N self-assembles into a helical capsid that accommodates the RNA genome to form a nucleocapsid, which protects the viral genome from host nucleases and serves as the template for viral replication. Both genome transcription and replication are carried out by the viral RNA-dependent RNA polymerase L and require the phosphoprotein P that bridges between the nucleocapsid and the polymerase. By obtaining atomic models for the authentic mumps virus nucleocapsid, we elucidate a concomitant conformational change that exposes the viral genome to its replication machinery. On the structural level, MuV nucleocapsids are templates for both viral transcription and replication.

Here, we isolated the authentic MuV nucleocapsids from stressed cells. After 1 h of 0.5 mM As(III) treatment, the isolated nucleocapsids were curved, similar to their intracellular morphology at early time points of stress but straightened on addition of the RNA-mimicking molecule heparin. We obtained two maps from subtomogram averaging on the heparin-straightened nucleocapsids isolated from cells after 1 h of 0.5 mM As(III) stress. The two maps exhibited distinctly different helical parameters: a 5.58 nm long-pitch structure constituting the majority class (77.7%) was resolved to 4.5 Å and a 4.70 nm short-pitch class (21.3%) was resolved to 6.3 Å. The RNA packaging of MuV follows the “rule of six,” i.e., six nucleotides per N subunit, and is coordinated by conserved residues from a loop containing Tyr350, Thr351, Arg354 in the upper CTD, and loop and helices containing Lys198, Arg194, Tyr260, Lys180 from the lower NTD. Interactions between subunits in consecutive turns of the nucleocapsid are mediated by the CTD-arm helix (a region succeeding the CTD), which inserts between the NTDs of two subunits in the upper turn. Within the same turn, domain swapping between the NTD arms (a region preceding the NTD) and CTD arms of consecutive subunits formed extensive contacts at the nucleocapsid lumen. Compared with the map of the majority class, density of this critical CTD-arm was missing in the map of the minority class indicating its high flexibility, as only full-length protein was detected by western blot analysis. In contrast, the loosely packed structure of the majority class exhibits higher exposure of the RNA on the nucleocapsid surface and higher likelihood for the unresolved C-terminal IDR of N protein to extend and interact with partner proteins, i.e., P and L, at the nucleocapsid surface.

> MSSVLKAFERFTIEQELQDRGEEGSIPPETLKSAVKVFVINTPNPTTRYQMLNFCLRIICSQNARASHRVGALITLFSLPSAGMQNHIRLADRSPEAQIERCEIDGFEPGTYRLIPNARANLTANEIAAYALLADDLPPTINNGTPYVHADVEGQPCDEIEQFLDRCYSVLIQAWVMVCKCMTAYDQPAGSADRRFAKYQQQGRLEARYMLQPEAQRLIQTAIRKSLVVRQYLTFELQLARRQGLLSNRYYAMVGDIGKYIENSGLTAFFLTLKYALGTKWSPLSLAAFTGELTKLRSLMMLYRDIGEQARYLALLEAPQIMDFAPGGYPLIFSYAMGVGTVLDAQMRNYTYARPFLNGYYFQIGVETARRQQGTVDNRVADDLGLTPEQRTEVTQLVDRLARGRGAGIPGGPVNPFVPPVQQQQPAAVYADIPALEESDDDGDEDGGAGFQNGVQVPAVRQGGQTDFRAQPLQDPIQAQLFMPLYPQVSNIPSNQNHQINRIGGLENQDLLRYNENGDSQQDARGEHGNTFPNNPNQNAQLQVGDWDE> RSTDTFNYATYHTLEEIYDFLDLLVAENPHLVSKIQIGNTYEGRPIYVLKFSTGGSKRPAIWIDTGIHSREWVTQASGVWFAKKITQDYGQDAAFTAILDTLDIFLEIVTNPDGFAFTHSTNRMWRKTRSHTAGSLCIGVDPNRNWDAGFGLSGASSNPCSETYHGKFANSEVEVKSIVDFVKDHGNIKAFISIHSYSQL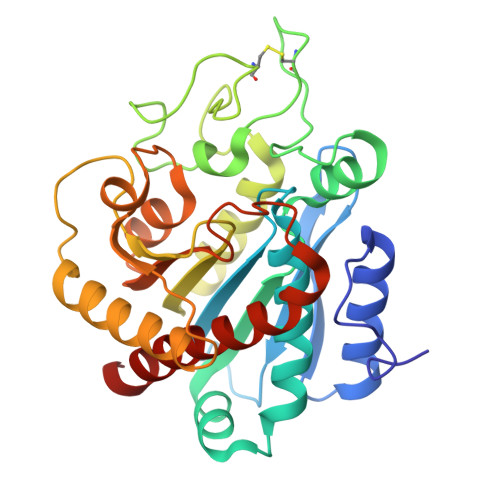LMYPYGYKTEPVPDQDELDQLSKAAVTALASLYGTKFNYGSIIKAIYQASGSTIDWTYSQGIKYSFTFELRDTGRYGFLLPASQIIPTAKETWLALLTIMEHTLNHP>[6x]MWKRSEQMKIKSGKCNMAAAMETEQLGVEIFETADCEENIESQDRPKLEPFYVERYSWSQLKKLLADTRKYHGYMMAKAPHDFMFVKRNDPDGPHSDRIYYLAMSGENRENTLFYSEIPKTINRAAVLMLSWKPLLDLFQATLDYGMYSREEELLRERKRIGTVGIASYDYHQGSGTFLFQAGSGIYHVKDGGPQGFTQQPLRPNLVETSCPNIRMDPKLCPADPDWIAFIHSNDIWISNIVTREERRLTYVHNELANMEEDARSAGV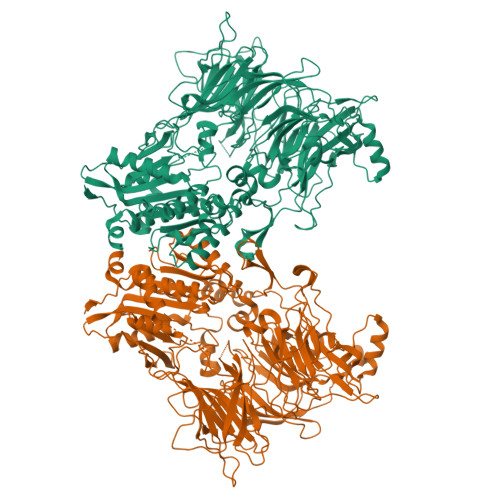ATFVLQEEFDRYSGYWWCPKAETTPSGGKILRILYEENDESEVEIIHVTSPMLETRRADSFRYPKTGTANPKVTFKMSEIMIDAEGRIIDVIDKELIQPFEILFEGVEYIARAGWTPEGKYAWSILLDRSQTRLQIVLISPELFIPVEDDVMERQRLIESVPDSVTPLIIYEETTDIWINIHDIFHVFPQSHEEEIEFIFASECKTGFRHLYKITSILKESKYKRSSGGLPAPSDFKCPIKEEIAITSGEWEVLGRHGSNIQVDEVRRLVYFEGTKDSPLEHHLYVVSYVNPGEVTRLTDRGYSHSCCISQHCDFFISKYSNQKNPHCVSLYKLSSPEDDPTCKTKEFWATILDSAGPLPDYTPPEIFSFESTTGFTLYGMLYKPHDLQPGKKYPTVLFIYGGPQVQLVNNRFKGVKYFRLNTLASLGYVVVVIDNRGSCHRGLKFEGAFKYKMGQIEIDDQVEGLQYLASRYDFIDLDRVGIHGWSYGGYLSLMALMQRSDIFRVAIAGAPVTLWIFYDTGYTERYMGHPDQNEQGYYLGSVAMQAEKFPSEPNRLLLLHGFLDENVHFAHTSILLSFLVRAGKPYDLQIYPQERHSIRVPESGEHYELHLLHYLQENLGSRIAALKVI> GPHMVIRAEKMEAVTHLAASISHEIRNPLTAARGFIQLIEEQPLAADKRRQYARIAIEELDRAEAIITDYLTFAKPAPETPEKLNVKLEIERVIDILRPLANMSCVDIQATLAPFSVIGEREKFRQCLLNVMKNAIEAMPNGGTLQVYVSIDNGRVLIRIADTGVGMTKEQLERLGEPYFTTKGVKGTGLGMMVVYRIIESMNGTIRIESEIHKGTTVSIY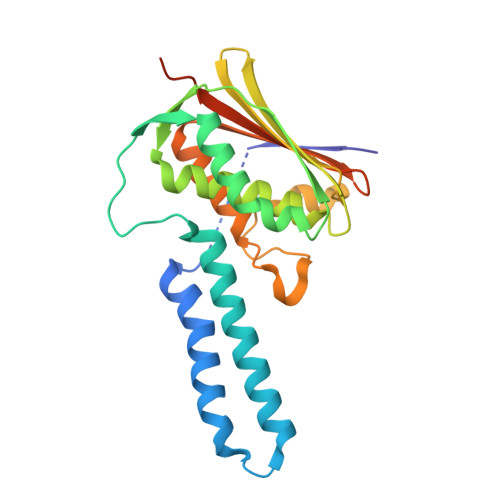LPLASSPSSSTISDKEKQLFAAL>[2x]ADKLFINALKKKFEESPEEKKTTFYTLGGWKQSERKTEFVNAGKEVAAKRGIPQYNPDIGTPLGQRVLMPYQVSTTDTYVEGDDLHFVNNAAMQQMWDDIRRTVIVGLNHAHAVIEKRLGKEVTPETITHYLETVNHAMPGAAVVQEHMVETHPALVADSYVKVFTGNDEIADEIDPAFVIDINKQFPEDQAETLKAEVGDGIWQVVRIPTIVSRTCDGATTSRWSAMQIGMSMISAYKQAAGEAATGDFAYAAKHAEVIHMGTYLPVRRARGENEPGGVPFGYLADICQSSRVNYEDPVRVSLDVVATGAMLYDQIWLGSYMSGGVGFTQYATAAYTDNILDDFTYFGKEYVEDKYGLCEAPNNMDTVLDVATEVTFYGLEQYEEYPALLEDQFGGSQRAAVVAAAAGCSTAFATGNAQTGLSGWYLSMYLHKEQHSRLGFYGYDLQDQCGASNVFSIRGDEGLP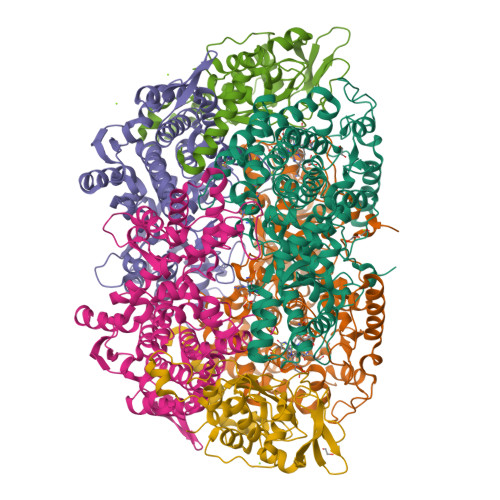LELRGPNYPNYAMNVGHQGEYAGISQAPHAARGDAFVFNPLVKIAFADDNLVFDFTNVRGEFAKGALREFEPAGERALITPAK;>AKFEDKVDLYDDRGNLVEEQVPLEALSPLRNPAIKSIVQGIKRTVAVNLEGIENALKTAKVGGPACKIMGRELDLDIVGNAESIAAAAKEMIQVTEDDDTNVELLGGGKRALVQVPSARFDVAAEYSAAPLVTATAFVQAIINEFDVSMYDANMVKAAVLGRYPQSVEYMGANIATMLDIPQKLEGPGYALRNIMVNHVVAATLKNTLQAAALSTILEQTAMFEMGDAVGAFERMHLLGLAYQGMNADNLVFDLVKANGKEGTVGSVIADLVERALEDGVIKVEKELTDYKVYGTDDLAMWNAYAAAGLMAATMVNQGAARAAQGVSSTLLYYNDLIEFETGLPSVDFGKVEGTAVGFSFFSHSIYGGGGPGIFNGNHIVTRHSKGFAIPCVAAAMALDAGTQMFSPEATSGLIKEVFSQVDEFREPLKYVVEAAAEIKNEI[2x];>AQYYPGTTKVAQNRRNFCNPEYELEKLREISDEDVVKILGHRAPGEEYPSVHPPLEEMDEPEDAIREMVEPIDGAKAGDRVRYIQFTDSMYFAPAQPYVRSRAYLCRYRGADAGTLSGRQIIETRERDLEKISKELLETEFFDPARSGVRGKSVHGHSLRLDEDGMMFDMLRRQIYNKDTGRVEMVKNQIGDELDEPVDLGEPLDEETLMEKTTIYRVDGEAYRDDVEAVEIMQRIHVLRSQGGFNLE[2x]> ICNGSLYPEPTLVPTPPPELPTDCGGPFELWEPNTTFSSTNFPNSYPNLAFCVWILNAQKGKNI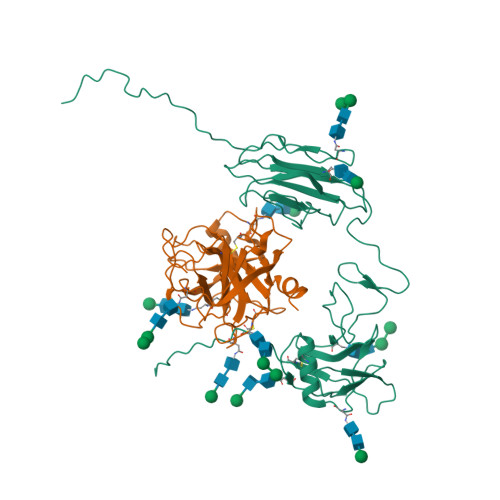QLHFQEFDLANINDVVEIRDGEEADSLLLAVYTGPGPVKDVFSTTNRMTVLLITNDVLARGGFKANFTTGYHLGIPEPCKADHFQCKNGECVPLVNLCDGHLHCEDGSDEADCVRFFNGTTNNNGLVRFRIQSIWHTACAENWTTQISNDVCQLLGLGSGNSSKPIFPTDGGPFVKLNTAPDGHLILTPSQQCLQDSLIRLQCNHKSCGKKLAAQDITPK;> IVGGSNAKEGAWPWVVGLYYGGRLLCGASLVSSDWLVSAAACVYGRNLEPSKWTAILGLHMKSNLTSPQTVPRLIDEIVINPHYNRRRKDNAIAMMHLEFKVNYTDYIQPICLPEENQVFPPGRNCSIAGWGTVVYQGTTANILQEADVPLLSNERCQQQMPEYNITENMICAGYEEGGIDSCQGDAGGPLMCQENNRWFLAGVTSFGYKCALPNRPGVYARVSRFTEWIQSFLH6-[4-[(7-chloranyl-1,2,3,4-tetrahydroacridin-9-yl)amino]butyl]-2-[(~{Z})-hydroxyiminomethyl]pyridin-3-ol 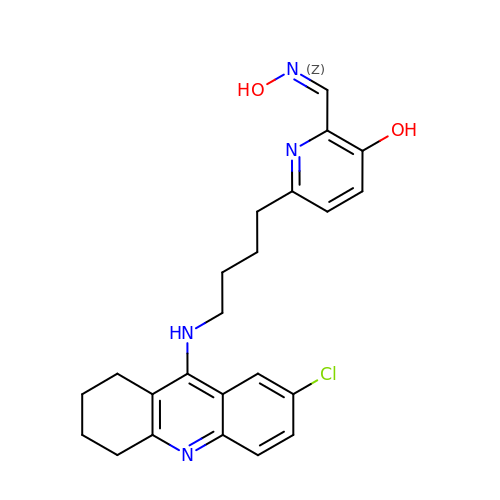| C23 H25 Cl N4 O2 | AEGVBHAVNJPGMI-WGARJPEWSA-N> AMDNYIYSIAHQLYEMYLQDED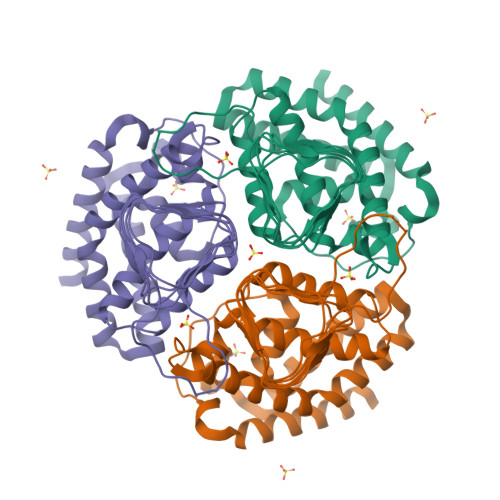AFHSKRDYPHKKVFTELQKLRKIFFPDFFMKHQKITESHIASELTKLVDYIKDSVTAYNDELFAHQCVMAILEKLPSIKRTLKTDLIAAYAGDPAAPGLSLIIRCYPGFQAVIVYRIAHVLYECGERYYCREMMESVHSYTSIDIHPGASIKGHFFIDHGVGVVIGETAIIGEWCRIYQSVTLGAMHFQEEGGVIKRGTKRHPTVGDYVTIGTGAKVLGNIIVGSHVRIGANCWIDRDVDSNQTVYISEHPTHFVKPCTTKGMKNDTEIIAIIPSSPLANSPSILEHHHHHH P2X receptors are trimeric cation channels that permeate a wide range of monovalent and divalent cations, by responding to extracellular ATP345. In the P2X receptors, each subunit has two transmembrane helices, connected by a relatively large extracellular domain. Seven subtypes of P2X receptors, named P2X1 to P2X7, are widely expressed in excitable and non-excitable cells, and are involved in diverse physiological processes such as muscle contraction, nociception, taste signal transduction and macrophage activation. While P2X receptors lack affinities for GTP and UTP, some P2X receptors have weak affinity for CTP (20 to 50 of times lower affinity than for ATP).

In this study, we determined the crystal structure of zebrafish P2X4 in complex with CTP, and conducted structure-based electrophysiological and spectroscopic analyses to reveal the mechanism underlying the nucleotide base specificity of P2X receptors. The subunit of CTP-bound structure is quite consistent with that of the previously determined ATP-bound structure, with root mean square deviation (RMSD) values below 0.4 Å for 324 Cα atoms, indicating that CTP can trigger the conformational changes similar to those by ATP. The overall structure forms a chalice-like shape assembled into a homotrimeric architecture, with a large extracellular domain and a small transmembrane domain, that is consistent with the previously determined P2X structures. The phosphate groups adopt a unique bent conformation and are directly recognized by the side chains of N296, R298, K316 from one subunit, and K70 and K72 from the adjacent subunit, consistent with the ATP-bound structure. The shape of the electron density for the base group was smaller than that in the ATP-bound structure, and could be readily assigned as the cytosine of the CTP molecule. While the side chain of the conserved threonine, T189, forms a hydrogen bond with the adenine ring in the ATP-bound structure, there is no equivalent hydrogen bond between the cytosine ring and the side chain of T189 in the CTP-bound structure. The O atom of the cytosine interacts with the side chain of R143, which had not been predicted in the previous superimposed model based on the ATP-bound structure. Furthermore, the NH2 atom of cytosine is recognized by the main chain carbonyl oxygen atoms of K70 and T189, as similarly observed in the ATP-bound structure, but their bond lengths seem to be 0.4–0.5 Å longer in the CTP-bound structure. Overall, the structural comparison between the CTP-bound and ATP-bound structures suggested that both CTP and ATP form three hydrogen bonds between their nucleotide bases and the receptor, but employ different residues. Therefore, the longer hydrogen bond lengths, rather than the difference in the number of hydrogen bonds, might be mainly responsible for the weaker affinity for CTP over ATP.

> GSSKKVGTLNRFTQALVIAYVIGYVCVYNKGYQDTDTVLSSVTTKVKGIALTKTSELGERIWDVADYIIPPQEDGSFFVLTNMIITTNQTQSKCAENPTPASTCTSHRDCKRGFNDARGDGVRTGRCVSYSASVKTCEVLSWCPLEKIVDPPNPPLLADAERFTVLIKNNIRYPKFNFNKRNILPNINSSYLTHCVFSRKTDPDCPIFRLGDIVGEAEEDFQIMAVRGGVMGVQIRWDCDLDMPQSWCVPRYTFRRLDNKDPDNNVAPGYNFRFAKYYKNSDGTETRTLIKGYGIRFDVMVFGQAGKFNIIPTLLNIGAGLALLGLVNVICDWIVLTFMK> MKIAVAGSGYVGLSLGVLLSLQNEVTIVDILPSKVDKINNGLSPIQDEYIEYYLKSKQLSIKATLDSKAAYKEAELVIIATPTNYNSRINYFDTQHVETVIKEVLSVNSHATLIIKSTIPIGFITEMRQKFQTDRIIFSPEFLRESKALYDNLYPSRIIVSCEENDSPKVKADAEKFALLLKSAAKKNNVPVLIMGASEAEAVKLFANTYLALRVAYFNELDTYAESRKLNSHMIIQGISYDDRIGMHYNNPSFGYGGYCLPKDTKQLLANYNNIPQTLIEAIVSSNNVRKSYIAKQIINVLKEQESPVKVVGVYRLIMKSNSDNFRESAIKDVIDILKSKDIKIIIYEPMLNKLESEDQSVLVNDLENFKKQANIIVTNRYD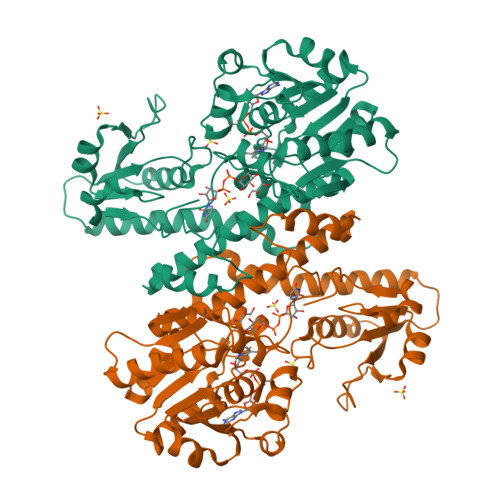NELQDVKNKVYSRDIFGRD> METQLQSIFEEVVKTEVIEEAFPGMFMDTPEDEKTKLISCLGAFRQFWGGLSQESHEQCIQWIVKFIHGQHSPKRISFLYDCLAMAVETGLLPPRLVCESLINSDTLEWERTQLWALTFKLVRKIIGGVDYKGVRDLLKVILEKILTIPNTVSSAVVQQLLAAREVIAYILERNACLLPAYFAVTEIRKLYPEGKLPHWLLGNLVSDFV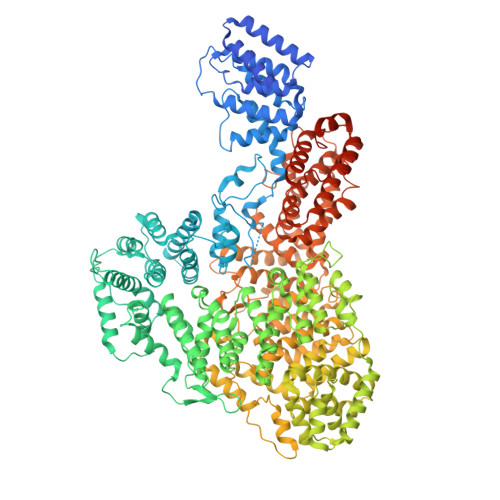DTFRPTARINSICGRCSLLPVVNNSGAICNSWKLDPATLRFPLKGLLPYDKDLFEPQTALLRYVLEQPYSRDMVCNMLGLNKQHKQRCPVLEDQLVDLVVYAMERSETEEKFDDGGTSQLLWQHLSSQLIFFVLFQFASFPHMVLSLHQKLAGRGLIKGRDHLMWVLLQFISGSIQKNALADFLPVMKLFDLLYPEKEYIPVPDINKPQSTHAFAMTCIWIHLNRKAQNDNSKLQIPIPHSLRLHHEFLQQSLRNKSLQMNDYKIALLCNAYSTNSECFTLPMGALVETIYGNGIMRIPLPGTNCMASGSITPLPMNLLDSLTVHAKMSLIHSIATRVIKLAHAKSSVALAPALVETYSRLLVYMEIESLGIKGFISQLLPTVFKSHAWGILHTLLEMFSYRMHHIQPHYRVQLLSHLHTLAAVAQTNQNQLHLCVESTALRLITALGSSEVQPQFTRFLSDPKTVLSAESEELNRALILTLARATHVTDFFTGSDSIQGTWCKDILQTIMSFTPHNWASHTLSCFPGPLQAFFKQNNVPQESRFNLKKNVEEEYRKWKSMSNENDIITHFSMQGSPPLFLCLLWKMLLETDHINQIGYRVLERIGARALVAHVRTFADFLVYEFSTSAGGQQLNKCIEILNDMVWKYNIVTLDRLILCLAMRSHEGNEAQVCYFIIQLLLLKPNDFRNRVSDFVKENSPEHWLQNDWHTKHMNYHKKYPEKLYFEGLAEQVDPPVQIQSPYLPIYFGNVCLRFLPVFDIVIHRFLELLPVSKSLETLLDHLGGLYKFHDRPVTYLYNTLHYYEMHLRDRAFLKRKLVHAIIGSLKDNRPQGWCLSDTYLKCAMNAREENPWVPDDTYYCRLIGRLVDTMAGKSPGPFPNCDWRFNEFPNPAAHALHVTCVELMALAVSGKEVGNALLNVVLKSQPLVPRENITAWMNAIGLIITALPEPYWIVLHDRIVSVISSPSLTSETEWVGYPFRLFDFTACHQSYSEMSCSYTLALAHAVWHHSSIGQLSLIPKFLTEVLLPIVKTEFQLLYVYHLVGPFLQRFQQERTRCMIEIGVAFYDMLLNVDQCSTHLNYMDPICDFLYHMKYMFTGDSVKEQVEKIICNLKPALKLRLRFITHISKMEPAAVPPQAMNSGSPAPQSNQVPVSLPVTQDVLFQGPGHHHHHH NrS-1 polymerase is a multidomain enzyme and is one key component of the phage replisome. The N-terminal Prim/Pol and HBD domains are responsible for DNA polymerization and de novo primer synthesis activities of NrS-1 polymerase. Here, we report two crystal structures, showing that NrS-1 CTR adopts one unique hexameric ring-shaped conformation. Although the central helicase domain of NrS-1 CTR shares structural similarity with the superfamily III helicases, the folds of the Head and Tail domains are completely novel.

Totally, two NrS-1 CTR structures were determined, one in A-form and another in B-form. The A-form crystals were grown in P212121 space group; per asymmetric unit contains six copies of NrS-1 CTR monomer, which were assembled into a ring-shaped architecture. NrS-1 CTR assembles into ring-shaped hexamer in both structures. The helicase domain forms hexameric ring in both A- and B-form NrS-1 CTR structures. NrS-1 CTR forms hexamer in both A- and B-form structures, however, as confirmed by the size-exclusion chromatographic analysis, NrS-1 N618 exists as a monomer.

>[6x]EEKDPLWLYKVLLTKGIEVWFDIKLEKYGIKRNNRVDYIAKSSLQQIVFEIIGKTPKNIAVPTYIGAYEPSKPEKWEEEGIKYINLFKPTPLMKVKPVKEMPEIVKNLLLNLFDYDAKSMGLFINWLAFIYQYKERTGVAWIFMGKQGTGKGLLVDLLKKIFEEHMSSNITDANLDSQFNPYLYNKLIVHLNEVSADNRKSRMLVKNRLKTWITDETLYINRKNMKEVEIKNFCNFIINSNETIPVDIEDSDRRFNVIECNNVLKEQEWWTTESYQEILNNAEGFAKYLAGIKVDRSKVNEVVMSEKKKAIVETTESVLKQIAKALTDRDIEWFLDNGLEGVVEKNIVNDFQWEELQEAITTGVIPNKYLMIIVEQILGDSKTITWIKRNIITPYQVGETTVVKMAGKPIRAIVVG>[2x]MSTNITFHASALTRSERTELRNQRGLTIWLTGLSASGKSTLAVELEHQLVRDRRVHAYRLDGDNIRFGLNKDLGFSEADRNENIRRIAEVAK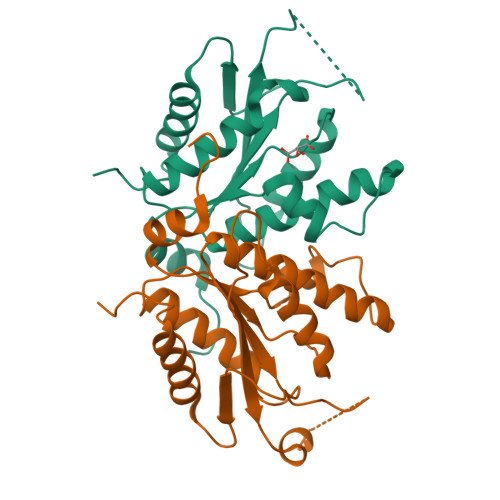LFADSNSIAITSFISPYRKDRDTARQLHEVATPGEETGLPFVEVYVDVPVEVAEQRDPKGLYKKAREGVIKEFTGISAPYEAPANPEVHVKNYELPVQDAVKQIIDYLDTKGYLPAKKE(1R,3R)-5-(2-((1R,3aS,7aR,E)-1-((R)-6-hydroxy-6-methylheptan-2-yl)-7a-methyloctahydro-4H-inden-4-ylidene)ethylidene)-2-methylenecyclohexane-1,3-diol | C27 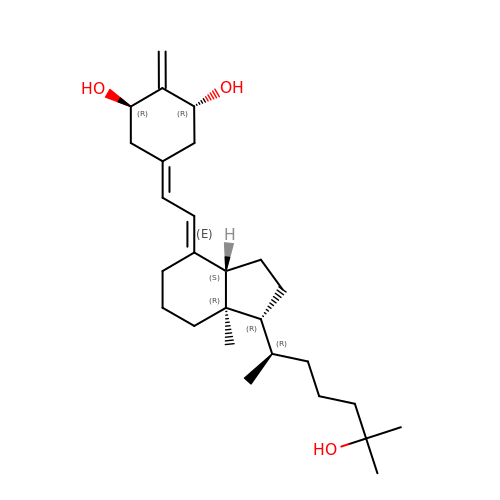H44 O3 | UHMPCVGLSKFXHR-JUTHDLPNSA-N> TIGMIALDAQGNLSGACTTSGMAYKMHGRVGDSPIIGA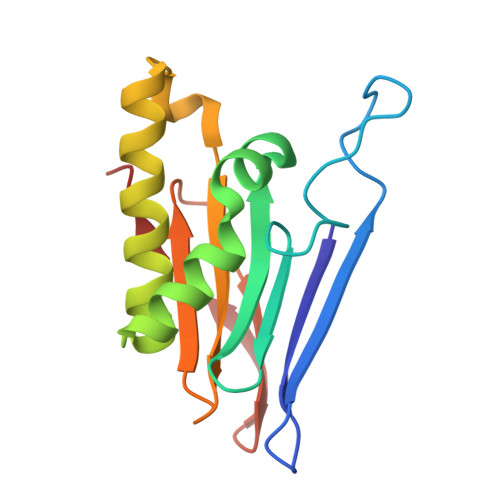GLFVDNEIGAATAIGHGEEVIRTVGTHLVVELMNQGRTPQQACKEAVERIVKIVNRRGKNLKDIQVGFIALNKKGEYGAYCIQDGFNFAVHDQKGNRLETPGFALK> MVKEFNTQTELSVRLEALWAVLSKDFITVVPKVLPHIVKDVQLIEGDGGVGTILIFNFLPEVSPSYQREEITEFDESSHEIGLQVIEGGYLSQ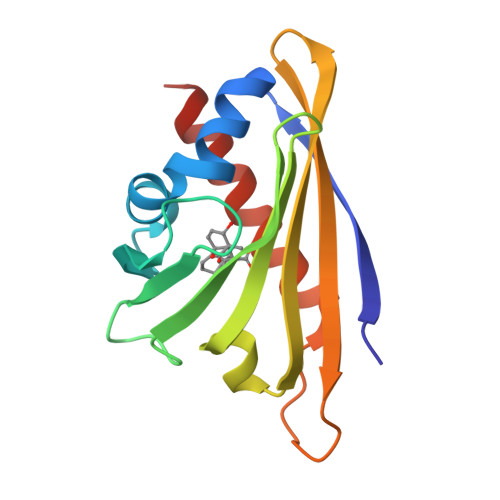GLSYYKTTFKLSEIEEDKTLVNVKISYDHDSDIEEKVTPTKTSQSTLMYLRRLERYLSNGSA> TLVHVASVEKGRSYEDFQKVYNAIALKLREDDEYDNYIGYGPVLVRLAWHISGTWDKHDNTGGSYGGTYRFKKEFNDPSNAGLQNGFKFLEPIHKEFPWISSGDLFSLGGVTAVQEMQGPKIPWRCGRVDTPEDTTPDNGRLPDADKDAGYVRTFFQRLNMNDREVVALMGAHALGKTHLKNSGYEGPGGAANNVFTNEFYLNLLNEDWKLEKNDANNEQWDSKSGYMMLPTDYSLIQDPKYLSIVKEYANDQDKFFKDFSKAFEKLLEDGI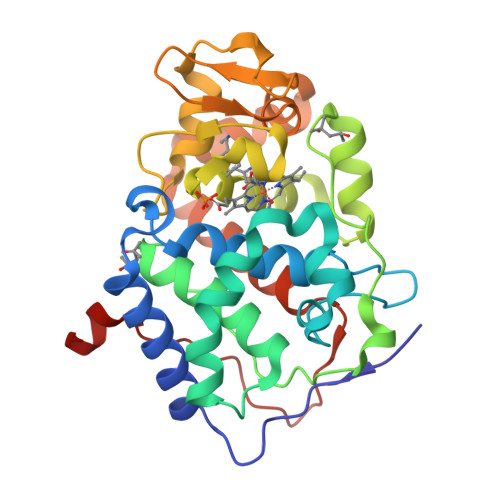TFPKDAPSPFIFKTLEEQGL>[2x]YKLSKLRTSTIMTDYNPNYSFAGKTSSISDLKEVPRKNITLIRGLGHGAFGEVYEGQVSGMPNDPSPLQVAVKTLPEVCSEQDELDFLMEALIISKFNHQNIVRCIGVSLQSLPRFILLELMAGGDLKSFLRETRPRPSQPSSLAMLDLLHV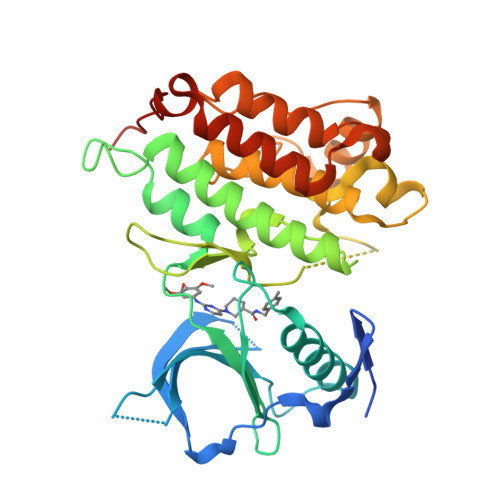ARDIACGCQYLEENHFIHRDIAARNCLLTCPGPGRVAKIGDFGMARDIYRASYYRKGGCAMLPVKWMPPEAFMEGIFTSKTDTWSFGVLLWEIFSLGYMPYPSKSNQEVLEFVTSGGRMDPPKNCPGPVYRIMTQCWQHQPEDRPNFAIILERIEYCTQDPDVINTALPIEYGPLVEEEEK>GHMPSAQIIDGKAIAAAIRSELKDKVAALRELYGGRVPGLASIIVGQRMDSKKYVQLKHKAAAEVGMASFNVELPEDISQEVLEVNVEKLNNDPNCHGIIVQLPLPKHLNENRAIEKIHPHKDADALLPVNVGLLHYKGREPPFTPCTAKGVIVLLKRCGIEMAGKRAVVLGRSNIVGAPVAALLMKENATVTIVHSGTSTEDMIDYLRTADIVIAAMGQPGYVKGEWIKEGAAVVDVGTTPVPDPSRKDGYRLVGDVCFEEAAARAAWISPVPGGVGPMTIAMLLENTLEAFKAALGVS[2x]

Three enzyme activities in the protozoan Leishmania major, namely N5,N10-methylenetetrahydrofolate dehydrogenase/N5,N10-methenyltetrahydrofolate cyclohydrolase (DHCH) and N10-formyltetrahydrofolate ligase (FTL) produce the essential intermediate N10-formyltetrahydrofolate. A two-step reaction follows, initially an NADP+ or NAD+ dependant oxidization of N5,N10-methylenetetrahydrofolate to the intermediate N5,N10-methenyltetrahydrofolate catalyzed by N5,N10-methylenetetrahydrofolate dehydrogenase (DH) and the methenyl derivative subsequently hydrolyzed to N10-formyltetrahydrofolate by N5,N10-methenyltetrahydrofolate cyclohydrolase (CH). All trypanosomatids possess this dehydrogenase and cyclohydrolase activity with a cytosolic bifunctional enzyme (DHCH). The cytosolic DHCH activity appears essential in L. major since knockouts of the disomic copies were not possible without ectopic expression of FTL to provide an alternative route to N10-formyltetrahydrofolate.

The crystal structure of LmDHCH has been determined at 2.7 Å resolution. The asymmetric unit is a homodimer and subunits are labeled A and B. The first and last few residues (1–2 and 1–3, 297–298 in chains A and B, respectively) are disordered and an additional three residues are disordered in chain B (248–250). Superposition of subunit A onto subunit B gives an RMSD of 1.7 Å over 286 main chain Cα atoms. This high value reflects differences in domain positions, which will be discussed, and in a loop adjacent to the active site (residues 240–255; RMSD 4.1 Å over 13 Cα). The LmDHCH subunit consists of 298 residues displaying a high level of secondary structure; 11 α-helices and 11 β-strands. The polypeptide folds into N- and C-terminal domains comprising residues 5–147 and 148–298, respectively. A cleft is formed between the two domains and at one end an NADP+ binding site, typical of a Rossmann fold (βαβαβ), is formed. The substrate-binding site is at the other end of the cleft. Analysis of the domains of LmDHCH from the crystallographically independent chains shows a significant pivot around a hinge (residues 150–152 and 274–280) with a rotation of almost 14° evident. The subunits appear in distinct states, with the active site slightly more compressed in one than the other and this may represent a feature of DHCH activity.>[2x]MKHHHHHHHMVSTLKPLKIGKHTIKFPIFQGGMGVGISWDELAGNVAKEGALGVISAVGTGYYKNMRFVERIVAKKPFEALNFYSKKALNEIFANARKICGNNPLGANILYAINDYGRVLRDSCEAGANIIITGAGLPTNMPEFAKDFSDVALIPIISSAKALKILCKRWSDRYKRIPDAFIVEGPLSGGHQGFKYEDCFKEEFRLENLVPKVVEASKEWGNIPIIAAGGIWDRKDIDTMLSLGASGVQMATRFLGTKECDAKVYADLLPTLKKEDILLIKSPVGYPARAINTGVIKRIEEGNAPKIACVSNCVAPCNRGEEAKKVGYCIADGLGRSYLGNREEGLYFTGANGYRVDKIISVHELIKELTEG;>[2x]GTSSMGYLMALFEDIQAVIAEQLNVDAAQVTPEAEFVKDLGADSLDVVELIMALEEKFGIEIPDEQAEKIVNVGDVVKYIEDNKLA

The bifunctional dehydrogenase/isomerase FabX is an essential UFA biosynthesis enzyme in the widespread human pathogen Helicobacter pylori, a bacterium etiologically related to 95% of gastric cancers. FabX belongs to the nitronate monooxygenase (NMO) flavoprotein family but contains an atypical [4Fe-4S] cluster absent in all other family members characterized to date. We demonstrate that the [4Fe–4S] cluster functions as a temporary electron depot that receives electrons from FMN and sends electrons back to FMN to achieve independent bidirectional internal electron transfer.

To investigate the acyl-ACP substrate recognition mechanism of FabX, we performed crystal screening of FabX–holo-ACP and FabX–octanoyl-ACP complexes under anaerobic condition which block dehydrogenation of the substrate (FabX requires oxygen for activity). We obtained crystal structures of FabX–holo-ACP complex at 2.8 Å resolution with space group P21 and FabX–octanoyl-ACP complex at 2.3 Å resolution with space group P212121. In contrast to the FabX–octanoyl-ACP complex, both of two FabX–holo-ACP complexes in the asymmetric unit were well determined and essentially identical (RMSD value of 0.4687). holo-ACP binds FabX predominantly through its α2-helix through electrostatic and hydrophobic interactions as expected. The PPant arm of holo-ACP stretches into the active tunnel of FabX, where it is stabilized through hydrophobic interactions with FabX residues including I147, S149, G184, and Y277. Moreover, the O40′ atom of the PPant arm forms an additional H-bond with the sidechain of E175. However, superposition of the FabX–holo-ACP complex with the FabX–octanoyl-ACP complex showed a surprising ~30° rotation between the ACP molecules of the two complexes. Specifically, holo-ACP rotates in the clockwise direction along the α2-helix with the sidechain of FabX R164 acting as the rotation fulcrum, allowing D35′ and D38′ from holo–ACP to form salt-bridges with the sidechain of FabX K152, which were not observed in the FabX–octanoyl-ACP complex. Moreover, the rotation weakens the interactions between α3-helix of octanoyl-ACP and FabX, and abolishes the interaction between D56′ of octanoyl-ACP and FabX T130.> DEAVVHDSYAFDKNQLIPVGARAEVGTTGYGGALLWQANPYVGLALGYNGG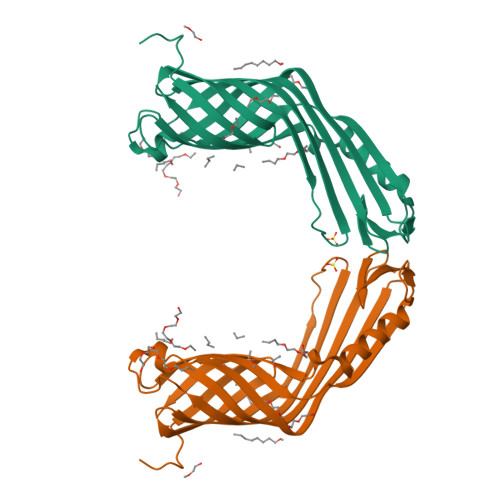DISWSDDVKVNGSTYDLDMDNNNVYLNAEIRPWGASTNRWAQGLYVAAGAAYLDNDYDLTRNVDATRSFRVNNQDFIAGADGVKINGQMSYKNDIAPYLGFGFAPKINKNWGVFGEVGAYYTGNPTVKLVSSGSAVTTGDQSLEEAVNAEARKIANDDKYKWLPVGKVGVNFFWGGHHHHHH> MASSRCPAPRGCRCLPGASLAWLGTVLLLLADWVLLRTALPRIFSLLVPTALPLLRVWAVGLSRWAVLWLGACGVLRATVGSKSENAGAQGWLAALKPLAAALGLALPGLALFRELISWGAPGSADSTRLLHWGSHPTAFVVSYAAALPAAALWHKLGSLWVPGGQGGSGNPVRRLLGCLGSETRRLSLFLVLVVLSSLGEMAIPFFTGRLTDWILQDGSADTFTRNLTLMSILTIASAVLEFVGDGIYNNTMGHVHSHLQGEVFGAVLRQETEFFQQNQTGNIMSRVTEDTSTLSDSLSENLSLFLWYLVRGLCLLGIMLWGSVSLTMVTLITLPLLFLLPKKVGKWYQLLEVQVRESLAKSSQVAIEALSAMPTVRSFANEEGEAQKFREKLQEIKTLNQKEAVAYAVNSWTTSISGMLLKVGILYIGGQLVTSGAVSSGNLVTFVLYQMQFTQAVEVLLSIYPRVQKAVGSSEKIFEYLDRTPRCPPSGLLTPLHLEGLVQFQDVSFAYPNRPDVLVLQGLTFTLRPGEVTALVGPNGSGKSTVAALLQNLYQPTGGQLLLDGKPLPQYEHRYLHRQVAAVGQEPQVFGRSLQENIAYGLTQKPTMEEITAAAVKSGAHSFISGLPQGYDTEVDEAGSQLSGGQRQAVALARALIRKPCVLILDDATSALDANSQLQVEQLLYESPERYSRSVLLITQHLSLVEQADHILFLEGGAIREGGTHQQLMEKKGCYWAMVQAPADAPE;> MRLPDLRPWTSLLLVDAALLWLLQGPLGTLLPQGLPGLWLEGTLRLGGLWGLLKLRGLLGFVGTLLLPLCLATPLTVSLRALVAGASRAPPARVASAPWSWLLVGYGAAGLSWSLWAVLSPPGAQEKEQDQVNNKVLMWRLLKLSRPDLPLLVAAFFFLVLAVLGETLIPHYSGRVIDILGGDFDPHAFASAIFFMCLFSFGSSLSAGCRGGCFTYTMSRINLRIREQLFSSLLRQDLGFFQETKTGELNSRLSSDTTLMSNWLPLNANVLLRSLVKVVGLYGFMLSISPRLTLLSLLHMPFTIAAEKVYNTRHQEVLREIQDAVARAGQVVREAVGGLQTVRSFGAEEHEVCRYKEALEQCRQLYWRRDLERALYLLVRRVLHLGVQMLMLSCGLQQMQDGELTQGSLLSFMIYQESVGSYVQTLVYIYGDMLSNVGAAEKVFSYMDRQPNLPSPGTLAPTTLQGVVKFQDVSFAYPNRPDRPVLKGLTFTLRPGEVTALVGPNGSGKSTVAALLQNLYQPTGGQVLLDEKPISQYEHCYLHSQVVSVGQEPVLFSGSVRNNIAYGLQSCEDDKVMAAAQAAHADDFIQEMEHGIYTDVGEKGSQLAAGQKQRLAIARALVRDPRVLILDEATSALDVQCEQALQDWNSRGDRTVLVIAHRLQTVQRAHQILVLQEGKLQKLAQL;> MSWALEMADTFLDNMRVGPRTYADVRDEINKRGREDREAARTAVHDPERPLLRSPGLLPEIAPNASLGVVHRRTGGTVTDSPRNPVTR

The transporter associated with antigen processing (TAP) transports these cytosolic peptides into the ER lumen, where a multi-component peptide-loading complex facilitates peptide-binding to nascent MHC-I molecules. TAP is an ER-resident transporter formed by two homologous subunits, TAP1 and TAP2. Similar to other ABC transporters, it contains two nucleotide-binding domains (NBDs) that hydrolyze ATP and two transmembrane domains (TMDs) that bind the substrate. For example, human herpes simplex virus (HSV) encodes the potent TAP inhibitor ICP47.

Here we present a 4.0 Å cryo-EM reconstruction of the human TAP/ICP47 complex and describe the specific atomic interactions that allow the viral peptide to bind tightly to TAP and lock it in an inactive state. With this map, we built and refined a model containing the 12 core TM-helices of TAP and the N-terminal 55 residues of ICP47. The 12 transmembrane (TM) helices at the core are arranged into two bundles, each consisting of TM 1–3 and 6 of one subunit and TM 4–5 of the other subunit. The N-terminal 55 residues of ICP47 form a helical hairpin structure, which inserts into the opening between the two TM bundles. The N-terminal 34 residues of ICP47 are largely buried inside the translocation pathway, forming a helical bundle with TAP2 TM helices 3 and 6. The last ordered residue of ICP47, P55, interacts with Y477, which normally makes an aromatic stacking interaction with the adenine ring of ATP. In TAP, however, this gating region is cracked open by ICP47 to a width approximately 4 Å in diameter. The presence of ICP47 blocks both openings; otherwise there would be a continuous pathway across the membrane, a state violating the alternating access model. In the TAP/ICP47 complex these residues are buried by ICP47, consistent with data showing that ICP47 precludes peptide binding. The strong interaction between ICP47 and TAP traps TAP in an inward-facing conformation with the two NBDs separated, unable to progress to the NBD-closed conformation necessary for ATP hydrolysis.>GHMADKIKDAKIIFVVGGPGSGKGTQCEKVVAKYGYTHLSSGDLLRAEVSSGSERGKQLQAIMQKGELVPLDTVLDMIKDAMIAKADVSKGYLIDGYPREVKQGEEFEKKIGKPCLLLYVDAKGETMVKRLMKRG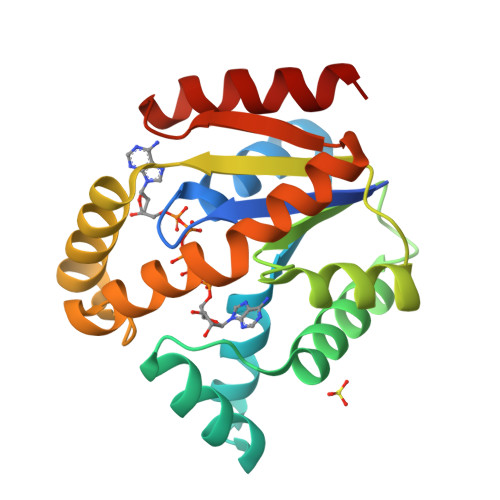ETSGRADDNEETIKKRLDLYYKATEPVIAFYEGRGIVRKVDSELPVDEVFKQVSTAIDAL[2x]>MKVPEAAISRLITYLRILEELEAQGVHRTSSEQLGGLAQVTAF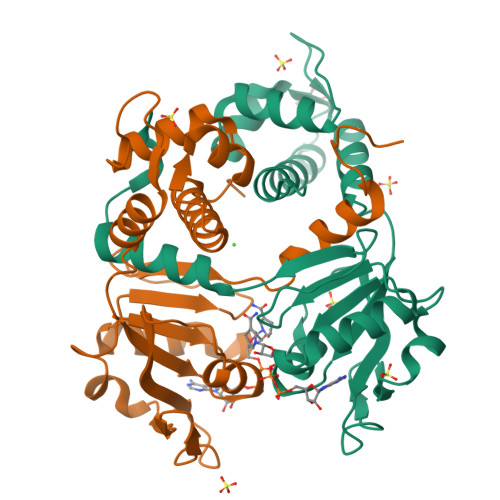QVRKDLSYFGSYGTRGVGYTVPVLKRELRHILGLNRKWGLCIVGMGRLGSALADYPGFGESFELRGFFDVDPEKVGRPVRGGVIEHVDLLPQRVPGRIEIALLTVPREAAQKAADLLVAAGIKGILNFAPVVLEVPKEVAVENVDFLAGLTRLSFAILNPKWREEMMG[2x]One such T6SS effector is Tlde1a from Salmonella Typhimurium. Tlde1a functions as an LD-carboxypeptidase to cleave tetrapeptide stems and as an LD-transpeptidase to exchange the terminal D-alanine of a tetrapeptide stem with a noncanonical D-amino acid. Our structural data revealed that Tlde1a possesses a unique LD-transpeptidase fold consisting of a dual pocket active site with a capping subdomain. This includes an exchange pocket to bind a D-amino acid for exchange and a catalytic pocket to position the D-alanine of a tetrapeptide stem for cleavage.

To probe the molecular features of Tlde1a that may contribute to this activity, we soaked Tlde1a crystals with D-Ala and D-Met. We were able to obtain cocrystal structures of Tlde1a in complex with each amino acid. The interaction of both D-amino acids with Tlde1a is facilitated by a salt bridge between the D-amino acid carboxylic acid and the sidechain of R115. Additional H-bonding to the carboxylic acid group is provided by the backbone amides of D40 and G116. Finally, the amide group of the D-amino acid participates in a bifurcated hydrogen bond with the acidic sidechain of D40, a water molecule, and a carbonyl of the Tlde1a His-tag cloning artifact. Moreover, in the Tlde1a native structure, the D-amino acid binding pocket is occupied by a sulfate from the crystallization condition, supporting the observation that H-bonds are the primary mode of ligand binding. It is also important to note that the Tlde1a complex with D-Ala contains a second bound D-Ala. However, this D-Ala is at a crystal packing interface, interacts with unconserved residues, and shows a poorer fit to the electron density. Taken together, these observations suggest that Tlde1a contains a D-amino acid binding pocket that may have no sidechain selectivity for the D-amino acid to be exchanged.

> MMAVRLTFDGQKLTWPGIGIFKATTGLPDLQWPDKQCVPDAAIPEGNYKLFIQFQGEAPIRNAADCDLGPSWGWSTIPRGQAAGTCEIYWANWGYNRIRLESADEKTRKACGGKRGGFYIHDSTKGYSHGCIEVEPVFFRILKQETEKENGEKTFTVNVKYVSGQQTNGGTKQG;> EHHHHHH>NAMVVTLD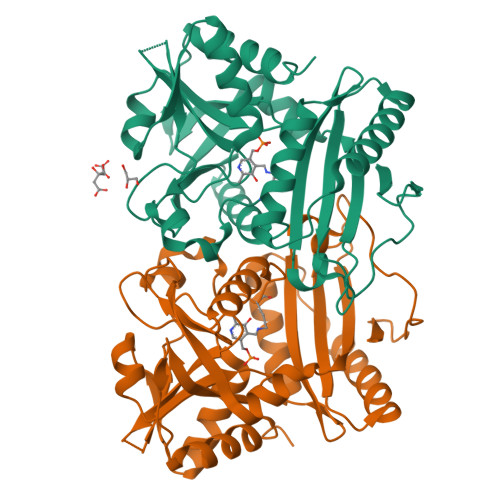GEILQPGMPLLHADDLAAVRGDGVFETLLVRDGRACLVEAHLQRLTQSARLMDLPEPDLPRWRRAVEVATQRWVASTADEGALRLIYSRGREGGSAPTAYVMVSPVPARVIGARRDGVSAITLDRGLPADGGDAMPWLIASAKTLSYAVNMAVLRHAARQGAGDVIFVSTDGYVLEGPRSTVVIATDGDQGGGNPCLLTPPPWYPILRGTTQQALFEVARAKGYDCDYRALRVADLFDSQGIWLVSSMTLAARVHTLDGRRLPRTPIAEVFAELVDAAIVSDR[4x]> ASTT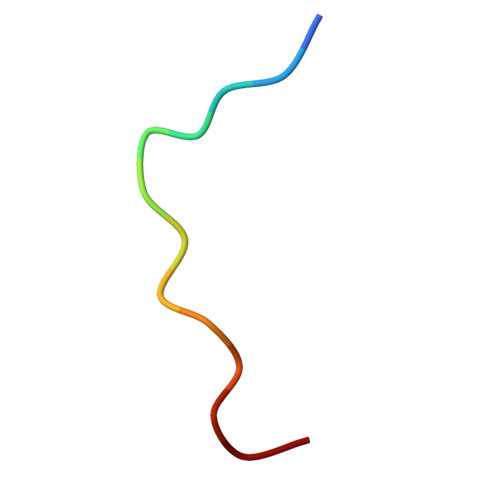GANSQRGSG>MALVDGFLELERSSGKLEWSAILQKMASDLGFSKILFGLLPKDSQDYENAFIVGNYPAAWREHYDRAGYARVDPTVSHCTQSVLPIFWEPSIYQTRKQHEFFEEASAAGLVYGLTMPLHGARGELGALSFSVEAENRAEANRFMESVLPTLWMLKDYALQSGAG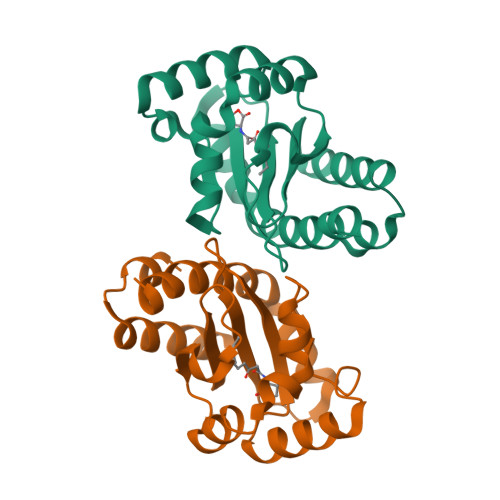LAFEHPVSKPVVLTSREKEVLQWCAIGKTSWEISVICNCSEANVNFHMGNIRRKFGVTSRRVAAIMAVNLGLITL[2x]> GSHMLSDEQMQIINSLVEAHHKTYDDSYSDFVRFRPPVREGPVTRSASRAASLHSLSDASSDSFNHSPESVDTKLNFSNLLMMYQDSGSPDSSEEDQQSRLSMLPHLADLVSYSIQKVIGFAKMIPGFRDLTAEDQIALLKSSAIEIIMLRSNQSFSLEDMSWSCGGPDFKYCINDVTKAGHTLELLEPLVKFQVGLKKLKLHEEEHVLLMAICLLSPDRPGVQDHVRIEALQDRLCDVLQAYIRIQHPGGRLLYAKMIQKLADLRSLNEEHSKQYRSLSFQPEH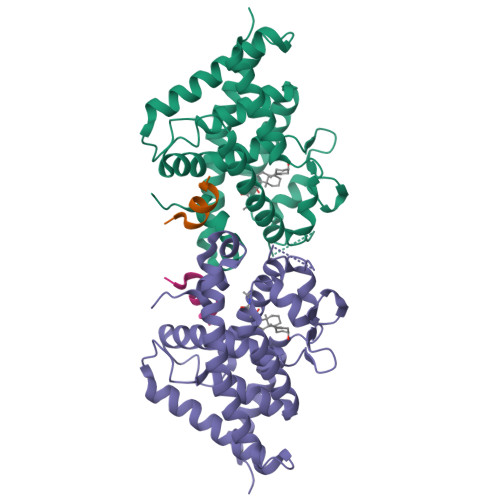SMQLTPLVLEVFGSEVS;> RHKILHRLLQEGSPS> SDPDPLQDFCVADLDGKAVSVNGHTCKPMSEAGDDFLFSSKLTKAGNTSTPNGSAVTELDVAEWPGTNTLGVSMARVDFAPGGTNPPHIHPRATEIGMVMKGE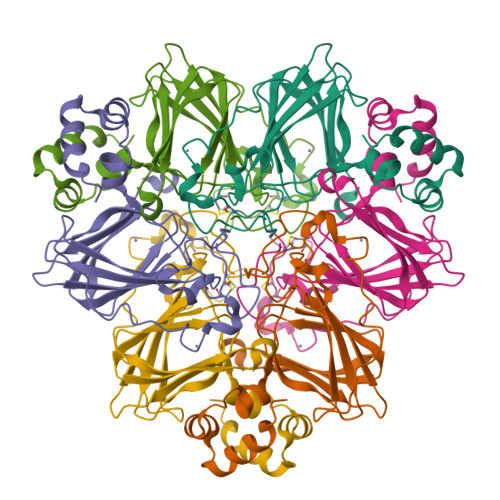LLVGILGSLDSGNKLYSRVVRAGETFVIPRGLMHFQFNVGKTEAYMVVSFNSQNPGIVFVPLTLFGSDPPIPTPVLTKALRVEAGVVELLKSKFAGGS>[2x]VGPKTGEENQVLVPNLNPTPENLEVVGDGFKI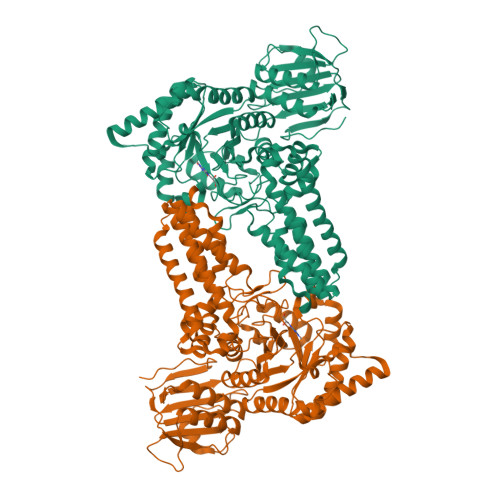TSSINLVGEEEADENAVNALREFLTANNIEINSENDPNSTTLIIGEVDDDIPELDEALNGTTAENLKEEGYALVSNDGKIAIEGKDGDGTFYGVQTFKQLVKESNIPEVNITDYPTVSARGIVEGFYGTPWTHQDRLDQIKFYGENKLNTYIYAPKDDPYHREKWREPYPESEMQRMQELINASAENKVDFVFGISPGIDIRFDGDAGEEDFNHLITKAESLYDMGVRSFAIYWDDIQDKSAAKHAQVLNRFNEEFVKAKGDVKPLITVPTEYDTGAMVSNGQPRAYTRIFAETVDPSIEVMWTGPGVVTNEIPLSDAQLISGIYNRNMAVWWNYPVTDYFKGKLALGPMHGLDKGLNQYVDFFTVNPMEHAELSKISIHTAADYSWNMDNYDYDKAWNRAIDMLYGDLAEDMKVFANHSTRMDNKTWAKSGREDAPELRAKMDELWNKLSSKEDASALIEELYGEFARMEEACNNLKANLPEVALEECSRQLDELITLAQGDKASLDMIVAQLNEDTEAYESAKEIAQNKLNTALSSFAVISEKVAQSFIQEALSFDLTLI>NNTLWTGPKPEANCIIEYGKQNPDSKLTLILVKNGGIVNGYVTLMGASDYVNTLFKNKNVSINVELYFDATGHILPDSSSLKTDLELKYKQTADFSARGFMPSTTAYPFVLPNAGTHNENYIFGQCYYKASDGALFPLEVTVMLNKRLPDSRTSYVMTFLWSLNAGLAPETTQATLITSPFTFSYIRED[3x];>[2x]PVFTQDVFVGSVEELSAAHTLVMKINATDADEPNTLNSKISYRIVSLEPAYPPVFYLNKDTGEIYTTSVTLDREEHSSYTLTVEARDGNGEVTDKPVKQAQVQIRILDVNDNIPVVENKVLEGMVEENQVNVEVTRIKVFDADEIGSDNWLANFTFASGNEGGYFHIETDAQTNEGIVTLIKEVDYEEMKNLDFSVIVANKAAFHKSIRSKYKPTPIPIKVKVK

The first step of adenoviral replication involves the interaction of the fibre protein and more precisely the globular trimeric knob with an attachment receptor from the host cell. Desmoglein 2 (DSG2), a newly identified adenovirus receptor has been reported to be used by some species B human adenoviruses including HAd3, HAd7, HAd11 and HAd14 for cell infection. The intermediate portion of the DSG2 ectodomain, consisting of EC2 and EC3, has been described as important for recognition by the HAd3 knob (HAd3K), the trimeric globular distal part of the fibre protein. Here, we report the structure of HAd3 fibre knob (HAd3K) in complex with one and two molecules of the DSG2 receptor.

A second minor complex harboring two receptors per trimeric fibre knob was also found. Different population of particles with either one or two EC2-EC3 modules (HAd3K/EC2-EC3 and HAd3K/(EC2-EC3)2) were identifiable in agreement with the 5.40S and 7.34S species previously reported. Their 3D structures were solved to an overall resolution of 3.5 and 3.8 Å, respectively. In the 2:1 complex (DSG2: trimeric knob), the interactions of the 1:1 complex are preserved, with the second DSG domain EC3 interacting with the G–H loop of monomer ‘A’ and the EC2 domain interacting with the A–B and C–D loop and N-terminal portion of the D strand of monomer ‘C’. In the 7.34S complex, one of the two EC2-EC3 modules is bound similarly to the corresponding one of the 5.40S complex. However, the relative positions of the modules differ slightly in the two cryo-EM maps (rmsd of 2.585 Å between the two EC2-EC3 modules) likely due to the binding of the second module in the 7.34S species. The main difference relies on three extra glutamates (E146-E268-E299) from HAd3K, which might be involved in the second module interaction while they do not participate to the first EC2-EC3 module binding. In the present structure, however, the interaction surfaces are different and the 1:1 and 1:2 binding modes are largely dictated by steric hindrance occurring close to the three-fold axis of the HAd3K, likely resulting in less favorable binding of two EC2-EC3 modules binding and extensive clashes if a third EC2-EC3 module is present. The structural data confirm the biochemical data since clashes occur with three modules excluding the more commonly observed three-receptor per knob binding mode observed for other HAd-receptor complexes. In addition, the non-classical stoichiometry of the HAd3K-DSG complex (1:1 and 1:2) results in non-symmetrical binding of the receptor to the trimeric knob.>MKKYIYIYFFFITITINDLVINNTSKCVSIERRKNNAYINYGIGYNGPDNKITKSRRCKRIKLCKKDLIDIGAIKKPINVAIFGSTGSIGTNALNIIRECNKIENVFNVKALYVNKSVNELYEQAREFLPEYLCIHDKSVYEELKELVKNIKDYKPIILCGDEGMKEICSSNSIDKIVIGIDSFQGLYSTMYAIMNNKIVALANKESIVSAGFFLKKLLNIHKNAKIIPVDSEHSAIFQCLDNNKVLKTKCLQDNFSKINNINKIFLCSSGGPFQNLTMDELKNVTSENALKHPKWKMGKKITIDSATMMNKGLEVIETHFLFDVDYNDIEVIVHKECIIHSCVEFIDKSVISQMYYPDMQIPILYSLTWPDRIKTNLKPLDLAQVSTLTFHKPSLEHFPCIKLAYQAGIKGNFYPTVLNASNEIANNLFLNNKIKYFDISSIISQVLESFNSQKVSENSEDLMKQILQIHSWAKDKATDIYNKHNSS[2x]

1-Deoxy-d-xylulose 5-phosphate reductoisomerase from Plasmodium falciparum (PfDXR or PfIspC) is a homodimeric enzyme, with each subunit consisting of 488 amino acid residues. The enzyme DXR is also known as IspC, derived from the gene name ispC in the isoprenoid biosynthesis pathway. It is the enzyme responsible for the second step of a six-step catalytic reaction sequence catalyzing the conversion of the substrate 1-deoxy-d-xylulose 5-phosphate (DOXP) to 2-C-methyl-d-erythritol 4-phosphate (MEP) in the non-mevalonate pathway (MEP pathway). Accordingly, DXR, which belongs to the MEP pathway, a metabolic pathway not present in mammals, is regarded as a promising target for drug discovery. For the catalytic function of DXR, one molecule of NADPH and one divalent metal ion (either Mn2+ or Mg2+) are required per subunit as cofactors.

The most notable feature of the MAMK218 complex was the observation of two distinct conformers for the N-phenylbutyl group of MAMK218, namely a bent and a curved conformer. Additionally, Trp296 exhibited two conformers, corresponding to the two conformers observed for MAMK218. The phenyl moiety of the N-phenylbutyl group was accommodated in the subpocket in the case of the bent conformer, whereas in the case of the curved conformer, it was located in the center of the active site cleft. The side chain of Trp296 involved in the recognition of the bent conformer of MAMK218 exhibited a similar conformation to that in the MAMK89 complex. The phenyl ring was in contact with the subpocket through vdW interactions with the side chains of Ser232, Pro358, and Pro363. Additionally, the phenyl ring was engaged in a CH-π interaction (T-shape stacking) with the imidazole ring of His341. In the case of MAMK218, the phenyl moiety of the N-phenylbutyl substituent was somewhat exposed to the protein surface, attributed to the two-carbon extension of the linker length of the N-substituent relative to MAMK150. Additionally, the terminal end of the N-phenylbutyl substituent in MAMK218 displayed a degree of flexibility. The temperature factor of the phenyl moiety of the N-phenylbutyl substituent in MAMK218 was higher than that of the core part of MAMK218, and the electron density of the phenyl moiety was found to be relatively weak. The residues 293-295 and 293-297, respectively, in the flexible loops of the ternary and quaternary complexes were observed to be disordered and, therefore, not modeled.> KVFERC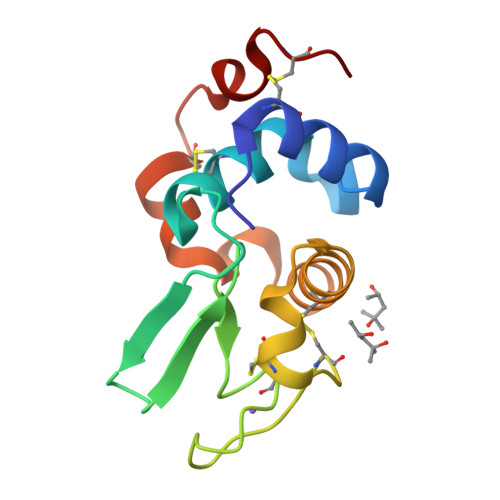ELARTLKKLGLDGYKGVSLANWLCLTKWESSYNTKATNYNPSSESTDYGIFQINSKWWCNDGKTPNAVDGCHVSCSELMENDIAKAVACAKHIVSEQGITAWVAWKSHCRDHDVSSYVEGCTL> HHHHHEETLLNTKLETADLKWVTFPQVDGQWEELSGLDEEQHSVRTYEVCDVQRAPGQAHWLRTGWVPRRGAVHVYATLRFTMLECLSLP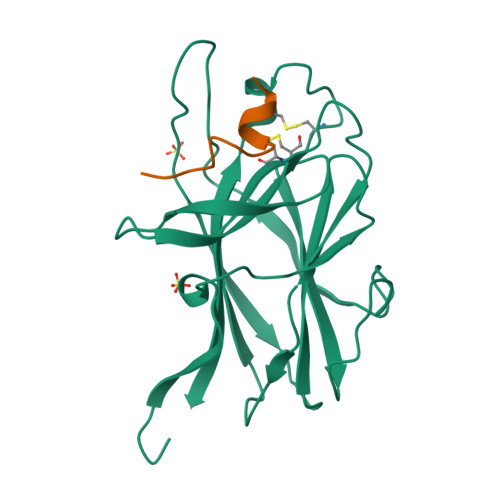RAGRSCKETFTVFYYESDADTATALTPAWMENPYIKVDTVAAEHLTRKRPGAEATGKVNVKTLRLGPLSKAGFYLAFQDQGACMALLSLHLFYKK;> TNYLFSPNGPIARAW>MSLTRDAASITPARVRAHVFRYPVSTPVKTSFGTMHDRPAVLVEVEDSDGAVGWGEVWCNFPACGAEHRARLVETVLAPLLTARAFADPAQAFAHLEARTAVLAIQTGEPGPLAQAIAGLDIALCDLAARRAGQPLWAWLGGSGDRIGVYASGINPENPEDVVARKAAEGYRAFKLKVGFDDARDVRNALHVRELLGAATPLMADANQGWDLPRARQMAQRLGPAQLDWLEEPLRADRPAAEWAELAQAAPMPLAGGENIAGVAAFETALAARSLRVMQPDLAKWGGFSGCLPVARAVVAAGLRYCPHYLGAGIGLQASAHLLAAVPGLASPGLLGVDANDNPLRSLLSPALATLHEGRITLGGAPGLGVTPDL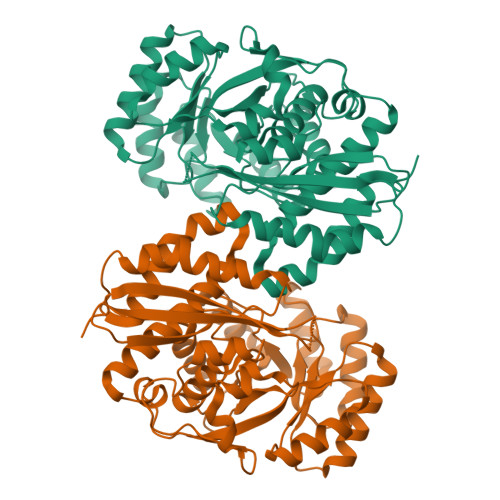AALRAACAAREGHHHHHH[4x]>MNLLDTLQRGLADLDAQGLRRVRRTADSACDAHMTVNGREIVGFASNDYLGLAAHPKLVAAFAEGAQRYGSGSGGSHLLGGHSRAHAKLEDELAGFAGGFSDAPRALYFSTGYMANLAAVTALAGKDATIFSDALNHASLIDGTRLSRATVQVYPHADTATLGALLEACTSQTKLIVTDTVFSMDGDIAPLAELLALAERHGAWLVVDDAHGFGVLGPQGRGALAAAALRSPHLVYVGTLGXAAGVAGAFVVAHETVIEWLIQRARSY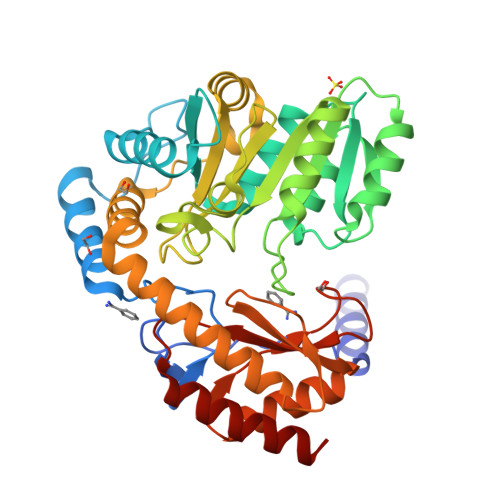IFTTAAPPAVAHAVSASLKVIAGDEGDARRAHLAALIERTRALLRRTRWQPVDSHTAVQPLVIGSNEATLAAMRALDAHGLWVPAIRPPTVPAGTSRLRISLSAAHSFDDLARLETALLRASEEA[3x]> GIGSILAETHGTRPDLTDQPIPDADYTWYTDGSSFLQEGQRRAGAAVTTETEVIWARALPAGTSAQRAELIALTQALKMAEGKKLNVYTDSRYAFATAHVHSEGREIKNKNEILALLKALF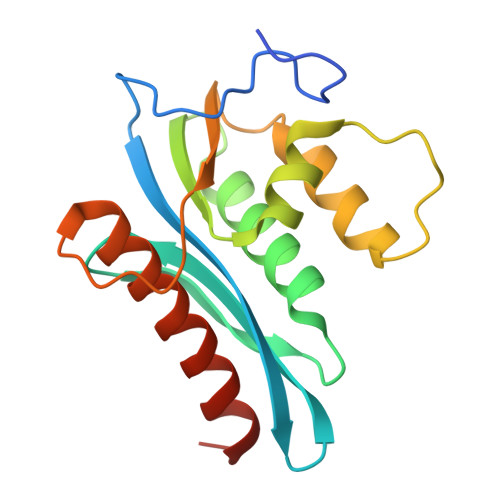LPKRLSIIHCPGHQKGNSAEARGNRMADQAAREAAMKAVLETSTLL>MPDIVNRKVEHVEIAAFENVDGLSSSTFLNDVILVHQGFPGI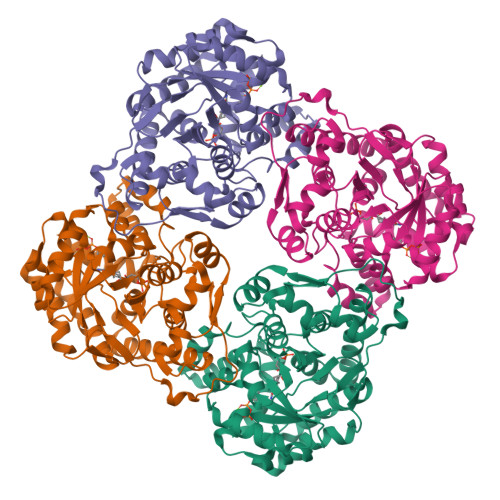SFSEINTKTKFFRKEISVPVMVTGMTGGRNELGRINKIIAEVAEKFGIPMGVGSQRVAIEKAEARESFAIVRKVAPTIPIIANLGMPQLVKGYGLKEFQDAIQMIEADAIAVHLNPAQEVFQPEGEPEYQIYALEKLRDISKELSVPIIVKESGNGISMETAKLLYSYGIKNFDTSGQGGTNWIAIEMIRDIRRGNWKAESAKNFLDWGVPTAASIMEVRYSVPDSFLVGSGGIRSGLDAAKAIALGADIAGMALPVLKSAIEGKESLEQFFRKIIFELKAAMMLTGSKDVDALKKTSIVILGKLKEWAEYRGINLSIYEKVRKRE[4x]>[6x]MAHHHHHHVGTGSNDDDDKAGLVEGQNYTVLANPIPQQQAGKVEVLEFFGYFCPHCAHLEPVLSKHAKSFKDDMYLRTEHVVWQKEMLTLARLAAAVDMAAA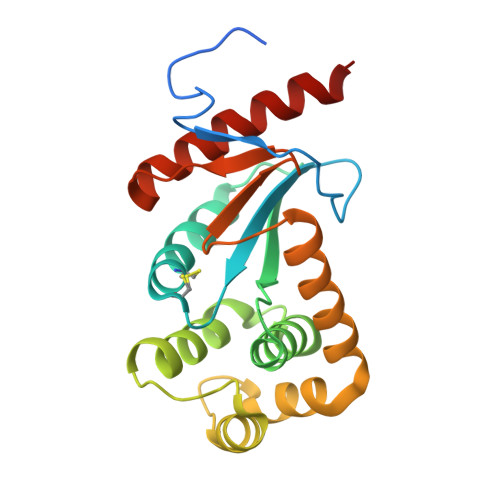DSKDVANSHIFDAMVNQKIKLQNPEVLKKWLGEQTAFDGKKVLAAYESPESQARADKMQELTETFQIDGTPTVIVGGKYKVEFADWESGMNTIDLLADKVREEQKAAQ> MMKLKSNQTRTYDGDGYKKRAACLCFRSESEEEVLLVSSSRHPDRWIVPGGGMEPEEEPSVAAVREVCEEAGVKGTLGRLVGIFENQERKHRTYVYVLIVTEVLEDWEDSVNIGRKREWFKIEDAIKVLQYHKPVQASYFETLRQGYSANNGTPVVATTYSVSAQS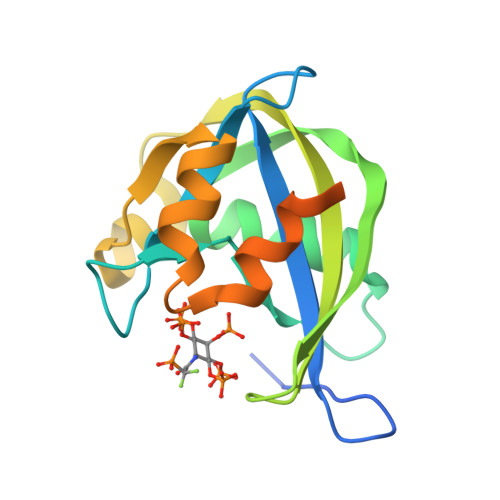SMSGIR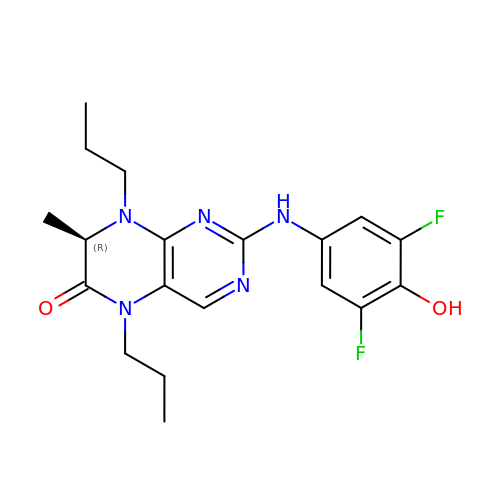(7R)-2-[(3,5-difluoro-4-hydroxyphenyl)amino]-7-methyl-5,8-dipropyl-7,8-dihydropteridin-6(5H)-one | C19 H23 F2 N5 O2 | OQSCAKQGDHBTSX-LLVKDONJSA-N>MAQIDFRKKINWHRRYRSPQGVKTEHEILRIFESDRGRIINSPAIRRLQQKTQVFPLERNAAVRTRLTHSMEVQQVGRYIAKEILSRLKELKLLEAYGLDELTGPFESIVEMSCLMHDIGNPPFGHFGEAAINDWFRQRLHPEDAESQPLTDDRCSVAALRLRDGEEPLNELRRKIRQDLCHFEGNAQGIRLVHTLMRMNLTWAQVGGILKYTRPAWWRGETPETHHYLMKKPGYYLSEEAYIARLRKELNLALYSRFPLTWIMEAADDISYCVADLEDAVEKRIFTVEQLYHHLHEA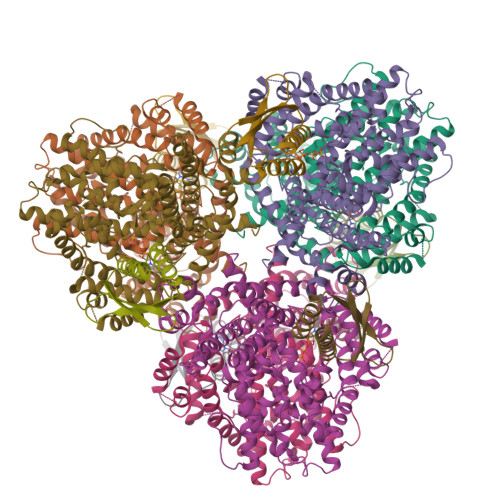WGQHEKGSLFSLVVENAWEKSRSNSLSRSTEDQFFMYLRVNTLNKLVPYAAQRFIDNLPAIFAGTFNHALLEDASECSDLLKLYKNVAVKHVFSHPDVERLELQGYRVISGLLEIYRPLLSLSLSDFTELVEKERVKRFPIESRLFHKLSTRHRLAYVEAVSKLPSDSPEFPLWEYYYRCRLLQDYISGMTDLYAWDEYRRLMAVEQ[6x];>[6x]GSFTMGRLYSGNLAAFKAATNKLFQLDLAVIYDDWYDAYTRKDCIRLRIEDRSGNLIDTSTFYHHDEDVLFNMCTDWLNHMYDQLKDWK> MENTENSVDSKSIKNLEPKIIHGSESMDSGISLDNSYKMDYPEMGLCIIINNKNFHKSTGMTSRSGTDVDAANLRETFRNLKYEVRNKNDLTREEIVELMRDVSKEDHSKRSSFVCVLLSHGEEGIIFGTNGPVDLKKIGNFFRGDRCRSLTGKPKLFI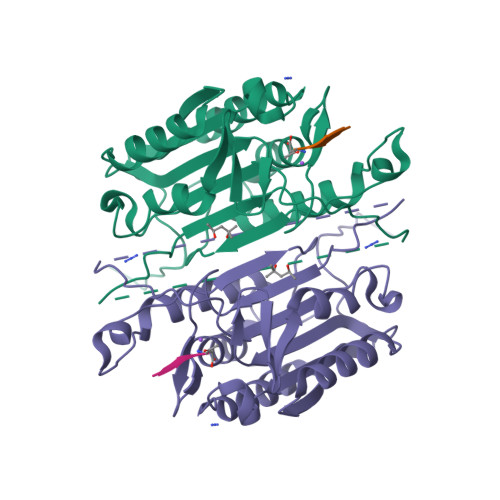IQACRGTELDCGIETDSGVDDDMACHKIPVEADFLYAYSTAPGYYSWRNSKDGSWFIQSLCAMLKQYADKLEFMHILTRVNRKVATEFESFSFDATFHAKKQIPCIHSMLTKELYFYHH>[3x]TTKKADYIWFNGEMVRWEDAKVHVMSHALHYGTSVFEGIRCYDSHKGPVVFRHREHMQRLHDSAKIYRFPVSQSIDELMEACRDVIRKNNLTSAYIRPLIFVGDVGMGVNPPAGYSTDVIIAAFPWGAYLGAEA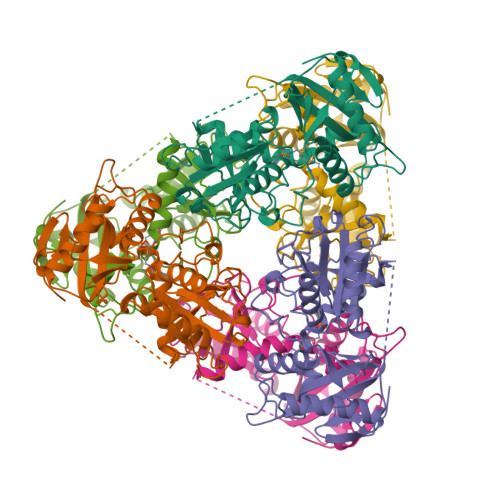LEQGIDAMVSSWNRAAPNTIPTAAKAGGNYLSSLLVGSEARRHGYQEGIALDVNGYISEGAGENLFEVKDGVLFTPPFTSSALPGITRDAIIKLAKELGIEVREQVLSRESLYLADEVFMSGTAAEITPVRSVDGIQVGEGRCGPVTKRIQQAFFGLFTGETEDKWGWLDQVNQ> MRPSALCLGGFTMKYKRGTGLWDEDHVNDFDAN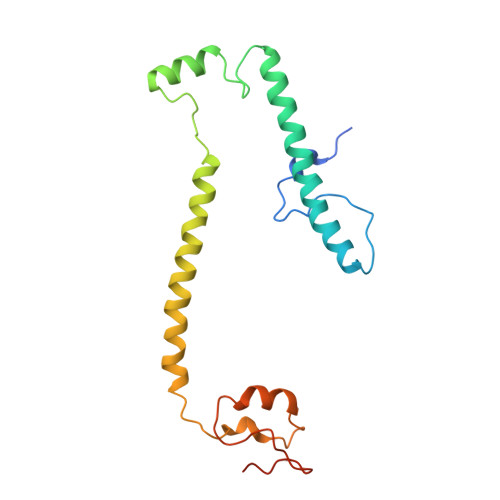KYLSARSTMRWYYGMERLQTRNNMNARRATQSYNNNMGLHHSGRGAFERELERRGIQVDKYPLTTTTGAARVAEMVLLRRQELEAHAKKAMESQRQARRRDAPSEWYDETEGPLNPRFLASMQSNYTQVITELPSSPVTGRRELPGASFA>[3x]GSHMGLTFNSNNICIDDNINTLWTGVNPTTANCQIMASSESNDCKLILTLVKTGALVTAFVYVIGVSNDFNMLTTHKNINFTAELFFDSTGNLLTSLSSLKTPLNHKSGQNMATGALTNAKGFMPSTTAYPFNVNSREKENYIYGTCYYTASDHTAFPIDISVMLNQRALNNETS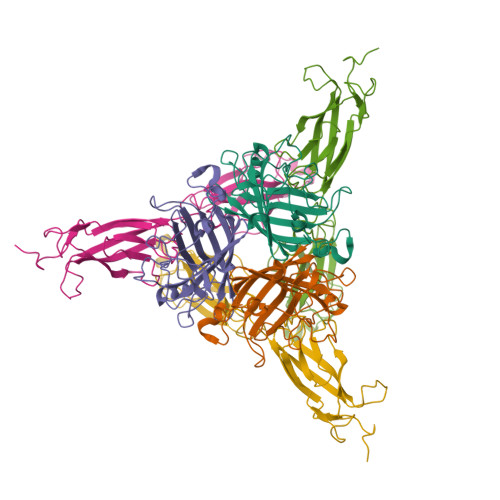YCIRVTWSWNTGVAPEVQTSATTLVTSPFTFYYIREDD;>QGAMEVLDINDNEPVFTQDVFVGSVEELSAAHTLVMKINATDADEPNTLNSKISYRIVSLEPAYPPVFYLNKDTGEIYTTSVTLDREEHSSYTLTVEARDGNGEVTDKPVKQAQVQIRILDVNDNIPVVENKVLEGMVEENQVNVEVTRIKVFDADEIGSDNWLANFTFASGNEGGYFHIETDAQTNEGIVTLIKEVDYEEMKNLDFSVIVANKAAFHKSIRSKYKPTPIPIKVKVKNVKEGI[3x]>MRKFILSLSILLSALLVACSSRNHYGDTGSLAGLQAMADSKYTRAQKKQKMGKIREMALKETALSVGAQAGLAWRAKIIDEQLNKQARNLDAIYDFNSLVLEHNILPPVLLEGRNTLNLADAQSIRISDRTYKVAKQAHFITTPPTWRQYLWMDYVKPEAPNVTLLPKTKAEKEIWCIYTERGWKNGIDQANTILEENIARIKEDFGGMILYRKLLAMNMVSPPYVSHTDLGVTGDGSEIHIDDRVLRITALPELNVNSAEWRAAVAKDENALERFKNMEKLANQAKIVITNKSWQPIIAPVS[13x];>[26x]MNNNKIVIMFIFSALLAGCAGTMKFKKPPINNPSDDATIKLAEAAVSVSDSMLEMAKVEKVITPPSKDNTLTIPNAYNLQARASVDWSGPIEELTARIAKAAHFRFRVLGKSPSVPVLISISTKDESLAEILRDIDYQAGKKASIHVYPNSQVVELRYAKIYS;>MMAEHDQNNDEYKFAELDSYDMDQAGESDLDSEASYQSGKEGLTKKKDIKRNALIAIGAVVFIMVMYKIIGWMFFSDKSSQVTSKPAIPPVTQVATPQPVQTIPTTTPIQQVQPTTIIEDDPDLKKKVSAIEMTQQSLRSEVNALSEQINAVNNNIKNLNAQIVNLNQIIGNMSNQIARQSEVINVLMARTTPKKVVKVSRPIVQARIIYYIQAVIPGRAWLIGSNGSTLTVREGSKIPGYGMVKLIDSLQGRILTSSGQVIKFSQEDS[31x];>[34x]MASKKENLKSLFSNTRTRVIIIFTAALLIIAVVIGFFKIRGATTGSIAAAEVSTVPGGIQSIPGVLDPTAQYAKLQEEQNITQAQVAEKTGGSAIPTIIRTQALGEGVGVIGSQSGVGFAALAQEELGGPQRSLWIQELQDGSCSKSVITKVVNQGAQLTDLKAACSCVQLKDSGYGLQELEQVCECKELKSAGYNARQLKEAGYSAGRLRNCGFDACELRNAGFTAQEMKDGGFSDGELKGAGFSDAEIAKASGLPDGITADDVRKAGCGAAALAKLRQAGVSASAIRKISGCTAEQLKAAGYTAKELKDAGFSAADLRRAGFSAAELKDAGFTARDLLNAGFTPADLAKAGFSDAQIKAAQAELPPGITPQDVKNAGCDVEALKKEREAGVSAALIRQYAGCSAQALKAAGFTDADLANAGFTPAQISAATPLSDAEIKAAGCDPDKLKKLFSAGVSAKRIKELNGCSAEALKAAGYDAQSLLAAGFTPQELLAAGFTPKQLEDAGLNPVSIIADGRVADCSVESLKKARAAGVSALTIKQTLGCSAAALKAAGYTAKELKDAGFTAAELKAAGFSAKELKDAGFTAKELRDAGFSAQELKDVGFSAKDLKDAGFSAAELKAAGFTAAQLKAAGFSAKDLKDAGFSAAELKAAGFSAKELKDAGFSASDLKNAGFSAKELKDAGFSASDLKSAGFSASELKNAGYSADELKKAGYTSAELRNAGFSPQESAVAGLQGPDLQQLDSSITGIPSIPGATPRPTTSDAASSAEQLQAILQKQNEQLAEQKYQQEIQQRTSDMLTAATQLVQDWKQVETQVYTEGTEETKTSGGESAVPGTGTGTGSNNQPVDQGAVSAQNQAIIKTGDIMFAVLDTSVNSDEPGPILATIVTGKLKGSKLIGSFNLPSNADKMVITFNTMSIPGAEKTISISAYAIDPNTARTALASRTNHHYLMRYGSLFASSFLQGFGNAFQSANTTITIGGTGGGNNITVANGVGRSTLENAVIGLATVGKAWSQQAQQLFNTPTTVEVYSGTGLGILFTQDVTTI;>[18x]MMKKYDQLCKYCLVIGLTFSMSCSIYAADQSDDAQQALQQLRMLQQKLSQNPSPDAQSGAGDGGDNAASDSTQQPNQSGQANAPAANQTATAGGDGQIISQDDAEVIDKKAFKDMTRNLYPLNPEQVVKLKQIYETSEYAKAATPGTPPKPTATSQFVNLSPGSTPPVIRLSQGFVSSLVFLDSTGAPWPIAAYDLGDPSSFNIQWDKTSNTLMIQATKLYNYGNLAVRLRGLNTPVMLTLIPGQKAVDYRVDLRVQGYGPNAKSMPTEEGIPPSANDLLLHVLEGVPPPGSRRLVVSGGDARAWLSNEKMYVRTNLTILSPGWLASMTSADGTHAYEMQKSPVLLVSWHGKVMQLKVEGL;>[13x]MRSLRTNYIYVLFKTTGLLFLLLLSACNRSGYIPENEVPKLPCRVDGACDATIIKMMTDLNKKGIKVASVGQNYLISIPASALFADQSPRLNWASYSLLNEIAAFLKQFRKIAITVTSYSSKYVSVKRERALTLARSRVVSEYLWSQGVDSRIIFTQGLGSDKPITSYTLGGDRSPNARVEITFRRAVA;>[13x]MRNLMRCLIMIKSLIKGVDMSRKLAKTRILGYGLMICFLAGCFHPPYNNFQPDRRAVKRVGVDTGIGAVAGAIASGTASGTLIGAAAGGTVGLVASIYRDSKRKIIRDLQKQDIQYVEYGDTRTLIIPTDKYFMFSSPRLNEICYPGLNNVIRLLNFYPQSTIYVAGFTDNVGSRSHKRKLSQAQAETMMTFLWANGIAAKRLKAEGYGDKNAISDNAIIHGSAQNRRIEIQWFTSPAQPPQPQMAYVK;>MLKRCYLLILLMFVLASCAHHKPQTPPAEVKKQGTSSTRQFRQVSSFNQIVVQGRLNVNLHTGYNKPEVMLRGDPRDLVQVRTIVKQNTLYVSLGQGYPDYGAVTVDIKTKFLNRFRYEGAGVVTGNNLRTSYLDLYLANEGTTRLAGNIGLQKLEAVGNGVTQINGVSSRNLQIVLKGDPKVLISGFVNLRQLDMYGKGTLSLYWIKSDTLTIRAKKAAKIQLAGIVNRLDVELWDFAQFKGKYLRAQRSFVKTHDKSVAEISAVNHQSSLATDASDIYYYNLSKTRADFMAFNGSVLDMREWGQSDLKDFDRYNKQFP[13x];>MLFLKIKTNQRTTMNILKPKAFLLASVFVLSISPAFAADGCCSKMGGINYCDSSAGRLVCNNGFYSTCYCTRHAVMDLQFLMGCCLWHGGVYPQLNSSGLVVCNDGYVSEECSLQKPVEQISVY[13x]

Legionella pneumophila is an opportunistic pathogen that causes the potentially fatal pneumonia known as Legionnaires’ disease. The pathology associated with infection depends on bacterial delivery of effector proteins into the host via the membrane spanning Dot/Icm type IV secretion system (T4SS). The Dot/Icm complex of L. pneumophila is one of the largest known T4SSs. The Dot/Icm T4SS has as many as 300 protein substrates, a striking contrast to the H. pylori Cag and B. pertussis Ptl T4SSs, each of which transports only one virulence factor.

Using 3D variability analysis, we reconstructed a total of five maps that displayed differences in the way the outer membrane cap (OMC) and periplasmic ring (PR) were positioned. These maps led to the identification of an approximate 16-fold symmetry about the center of the dome positioned within the OMC. Within this dome there are 16 α-helices that appear nearly identical at this resolution. Indeed, a model of the C-terminal domain of DotG generated in Swiss Model using VirB10 as a template fits into the resolved dome density (Waterhouse et al., 2018). However, we have unexpectedly uncovered that the Dot/Icm incorporates only 16 copies of DotG into the OMC dome out of the 18 DotG copies in the PR, giving rise to another symmetry mismatch within this system. Based on the structure of DotG modeled within the PR (residues 791–824) and the homology model fit into the dome density (consisting approximately of residues 857–1046), we hypothesize that DotG extends from the PR to the dome, though a physical connection between the two structures is not observed. (A) Two DotC were observed in the maps that were reconstructed during 3D variability analysis, one which contains an N-terminal extension (DotCLong) and one which does not (DotCshort). In contrast, the N-terminal extension of DotC was modeled as two relatively large helices positioned near DotG and bridging adjacent asymmetric units. Notably, this portion of DotC was only observed in either four or five of the 13 copies of DotC observed in each map. The movie shows that the OMC dome, OMC disk, and PR of Dot/Icm T4SS can accommodate various orientations in relation to each other that suggest that the complex could undergo a ratcheting motion, in which the dome and PR rotate back and forth about the central axis with the different regions of the complex tethered together by the physical connections across the symmetry mismatches.>ETTATTGIGVNFIGDSATECSFGIENTAGGSAVFHNYTRGASNSVTKNNQLLGGYGSRPWLGSTYTEHSNAALHFLGAGDTSATNHGGWIRLLVTPKGKTISDRVPAFRLSDNGDLWLVPDGAMHSDLGLVRSIETLNAAVPRFNAPSIQDGRGLKIVAPQAPEIDLIAPRGSGASAPAIRAMWCDGSLADTTRYIGATQPGSTFYIGASGHDGEKFDSMRGSVAIKSAGGWGPTSTPTQVVLETCESGSISRLPRWGVDHNGTLMPMADN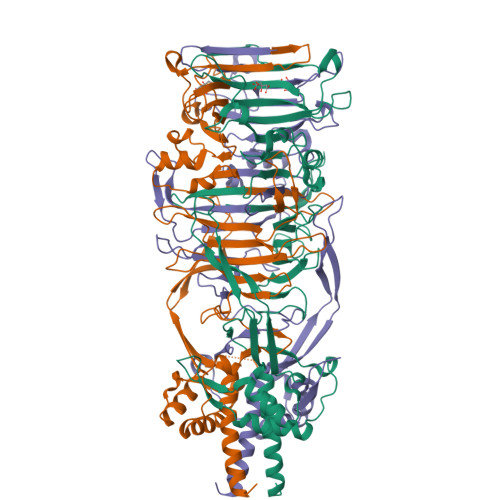RYNLGWGSGRVKQVYAVNGTINTADARLKNDVRAMSDPETEAAKAIAKEIGFWTWKEQADMNDIREHCGLTVQRAIEIMESFGLDPFKYGFICYDKWDEHTVVSEYGPANEDGTENPIYKTIPAGDHYSFRLEELNLFIAKGFEARLSAIEDKLGM[9x]>MGRDHRKIGKQLDLYHMQEEAPGMVFWHNDGWTIFRELEVFVRSKLKEYQYQEVKGPFMMDRVLWEKTGHWDNYKDAMFTTSSENREYCIKPMNCPGHVQIFNQGLKSYRDLPLRMAEFGSCHRNEPSGALHGLMRVRGFTQDDAHIFCTEEQIRDEVNACIRMVYDMYSTFGFEKIVVKLSTRPDKRIGSDEMWDRAEADLAVALEENNIPFEYQLGEGAFYGPKIEFTLYDCLDRAWQCGTVQLDFSLPSRLSASYVGEDNERKVPVMIHRAILGSMERFIGILTEEFAGFFPTWLAPVQVVVMNITD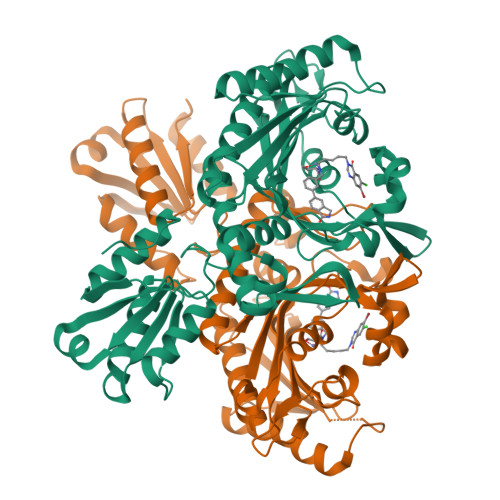SQSEYVNELTQKLQNAGIRVKADLRNEKIGFKIREHTLRRVPYMLVCGDKEVEAGKVAVRTRRGKDLGSLDVNDVIEKLQQEIRSRSLQQLEELEHHHHHH[2x]> GPVSSKEQTVETTGAEFRLRPEISVAQTDYGMVLLDGRSGEYWQLNDTAALIVQRLLDGHSPADVAQFLTSEYEVERTDAERDIAALVTSLKE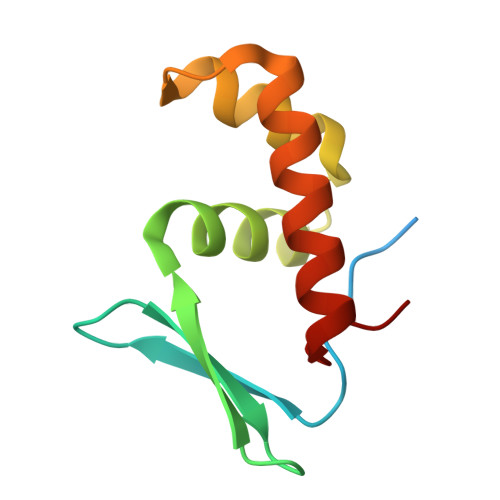NGMALP>[2x]MVLDNLGKALANTLKKIARASSVDEALIKELVRDIQRALIQADVNVRLVLQLTREIQRRALEEKPPAGISKKEHIIKIVYEELTKFLGTEAKPIEIKEKPTILLMVGIQGSGKTTTVAKLARYFQKRGYKVGVVCSDTWRPGAYHQLRQLLDRYHIEVFGNPQEKDAIKLAKEGVDYFKSKGVDIIIVDTAGRHKEDKALIEEMKQISNVIHPHEVILVIDGTIGQQAYNQALAFKEATPIGSIIVTKLDGSAKGGGALSAVAATGAPIKFIGTGEKIDDIEPFDPPRFVSRLLGLGDIQGLLEKFKELEKEVEIKEEDIERFLRGKFTLKDMYAQLEAMRKMGPLKQILRMIPGLGYSLPDDVISIGEERLKKFKVIMDSMTEEELLNPEIINYSRIKRIARGSGTSTKDVKELLDQYRQMKKLFKSMNKRQLSRLARRFGM

In all living cells the signal recognition particle (SRP) recognizes nascent polypeptides destined for secretion or membrane insertion as they emerge from translating ribosomes. As SRP binds to signal sequences emerging from the ribosomes, the resulting complex composed of the SRP and the ribosome-nascent chain complex is then targeted towards the membrane through the GTP-dependent interaction with the membrane-associated SRP receptor (SR also named FtsY in bacteria). We describe the X-ray structures of SRP54 and SRP19 the two protein constituting the proteinaceous core of the SRP from the hyperthermophilic archaeon Pyrococcus furiosus. SRP54 and SRP19 constitute the conserved core in all archaeal and eukaryotic SRPs.

Our structure of Pfu-SRP54 is the first full-length SRP54 structure bound to GDP. The protein interacts with the nucleotide through an intricate network of hydrogen bonds involving residues from the conserved motifs I, II, IV and V. The paired hydrogen bonds between the carboxylate group of Asp250 in motif IV and the N1 and N2- nitrogens of the guanine ring are canonical nucleotide-specificity determinant seen in all SRP-GTPases. In particular, the sidechains from glutamate Glu276 and Lys248 in motif IV sandwich the guanine and ribose moieties of GDP. Lys113 sidechain from the P-loop sits between the carboxylate headgroups of aspartates Asp137 (motif II) and Asp189 (motif III) near the β-phosphate of the GDP but does not interact with the GDP. The catalytic Asp137 is located 6.6 Å away from the β-phosphate of the GDP. Despite the presence of magnesium in the crystallization liquour there is no clear sign of magnesium ion bound next to the GDP molecule. The M domain of Pyrococcus furiosus appears as a stable and well-defined structural module with the exception of the finger loop (residues L346 to D363) that was not observed in the electron density maps. A groove flanked by helices α10, α11 and α14 and the finger loop constitutes the putative signal sequence binding site. Pfu-SRP54 appears as a flexible molecule with a stable though dynamic M domain articulated on a flexible linker that connects it to the NG catalytic core.> MEGSTGFDGDATTFFAPDAVFGDRVRRFQEFLDTFTSYRDSVRSIQVYNSNNAANYNDDQDDADERDLLGDDDGDDLEKEKKAASSTSLNILPHRIIISLDDLREFDRSFWSGILVEPAYFIPPAEKALTDLADSMDDVPHPNASAVSSRHPWKLSFKGSFGAHALSPRTLTAQHLNKLVSVEGIVTKTSLVRPKLIRSVHYAAKTGRFHYRDYTDATTTLTTRIPTPAIYPTEDTEGNKLTTEYGYSTFIDHQRITVQEMPEMAPAGQLPRSIDVILDDDLVDKTKPGDRVNVVGVFKSLGAGGMNQSNSNTLIGFKTLILGNTVYPLHARSTGVAARQMLTDFDIRNINKLSKKKDI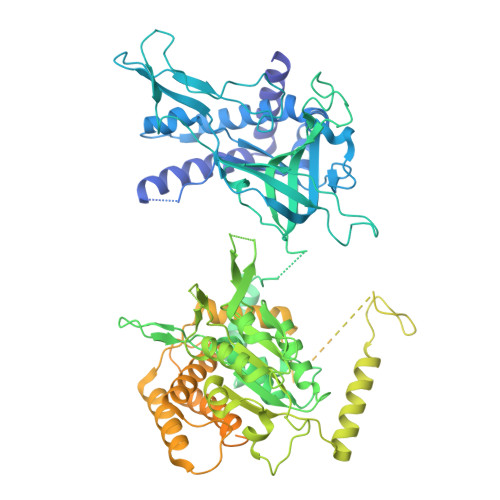FDILSQSLAPSIYGHDHIKKAILLMLMGGVEKNLENGSHLRGDINILMVGDPSTAKSQLLRFVLNTASLAIATTGRGSSGVGLTAAVTTDRETGERRLEAGAMVLADRGVVCIDEFDKMTDVDRVAIHEVMEQQTVTIAKAGIHTTLNARCSVIAAANPVFGQYDVNRDPHQNIALPDSLLSRFDLLFVVTDDINEIRDRSISEHVLRTHRYLPPGYLEGEPVRERLNLSLAVGEDADINPEEHSNSGAGVENEGEDDEDHVFEKFNPLLQAGAKLAKNKGNYNGTEIPKLVTIPFLRKYVQYAKERVIPQLTQEAINVIVKNYTDLRNDDNTKKSPITARTLETLIRLATAHAKVRLSKTVNKVDAKVAANLLRFALLGEDIGNDIDEEESEYEEALSKRSPQKSPKKRQRVRQPASNSGSPIKSTPRRSTASSVNATPSSARRILRFQDDEQNAGEDDNDIMSPLPADEEAELQRRLQLGLRVSPRRREHLHAPEEGSSGPLTEVGTPRLPNVSSAGQDDEQQQSVISFDNVEPGTISTGRLSLISGIIARLMQTEIFEEESYPVASLFERINEELPEEEKFSAQEYLAGLKIMSDRNNLMVADDKVWRV2-{[(2E)-but-2-enoyl]amino}-2-deoxy-beta-D-glucopyranose 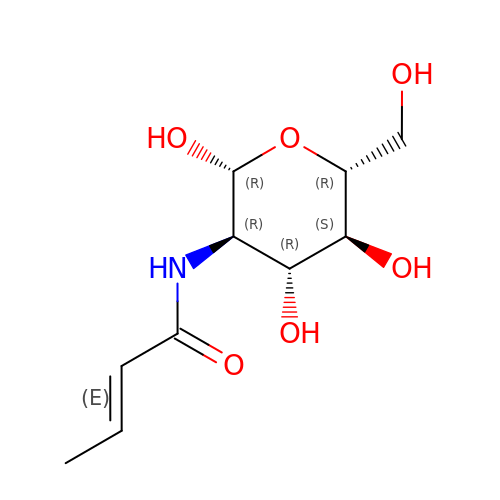| C10 H17 N O6 | GANGCWNSYXFAHD-SUZWSAGVSA-N~{N}-[(1~{S})-2-azanyl-1-[5-(hydroxymethyl)-1,3-thiazol-2-yl]ethyl]-3-methyl-5-[5-(trifluoromethyl)pyridin-2-yl]-1~{H}-pyrrole-2-carboxamide 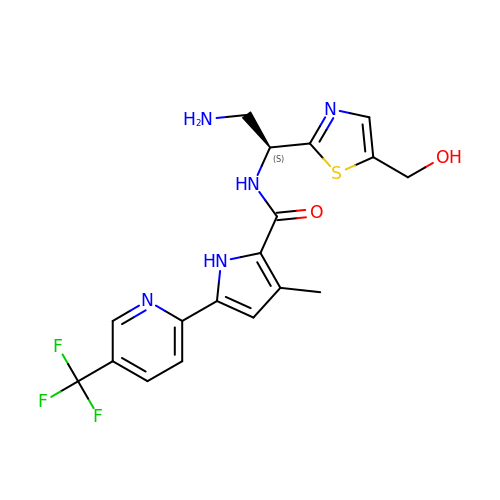| C18 H18 F3 N5 O2 S | BILBXEUAJZPBIW-AWEZNQCLSA-N6-(2-methoxyphenyl)-N~4~,N~4~-bis[(pyridin-2-yl)methyl]pyrimidine-2,4-diamine 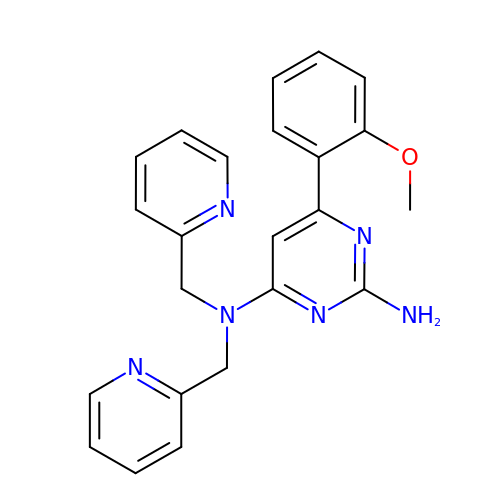| C23 H22 N6 O | BOPSVMQMLOGQBG-UHFFFAOYSA-N>GTTSQKHRDFVTEPMGEKPVGSLAGIGEVLGKKLEERGFDKAYVVLGQFLVLKKDEDLFREWLKDTAGANAKQSRDAFGALREWADAFL[4x];>[2x]GGGSVTKKRKLESTESRSSFSQHARTSGRVAVEEVDEEGKFVRLRNKSNEDQSMGNWQIKRQNGDDPLLTYRFPPKFT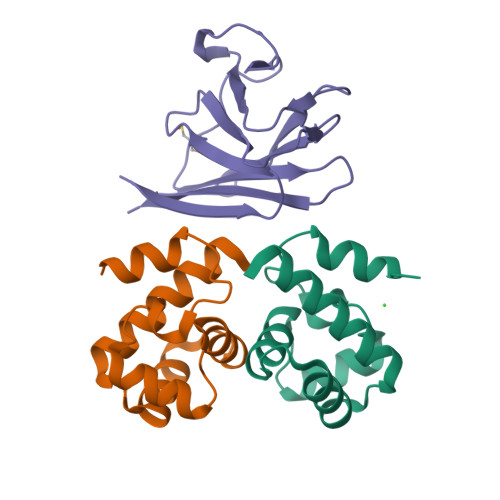LKAGQVVTIWAAGAGATHSPPTDLVWKAQNTWGCGNSLRTALINSTGEEVAMRKLVRSVTVVEDDEDEDGDDLLHHHH> AGCATGA;> TACTGACTCATGC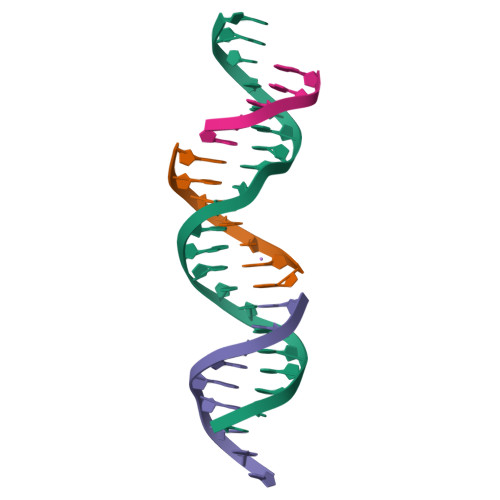TCATCTGA;> TATCAGATG;> GTCAG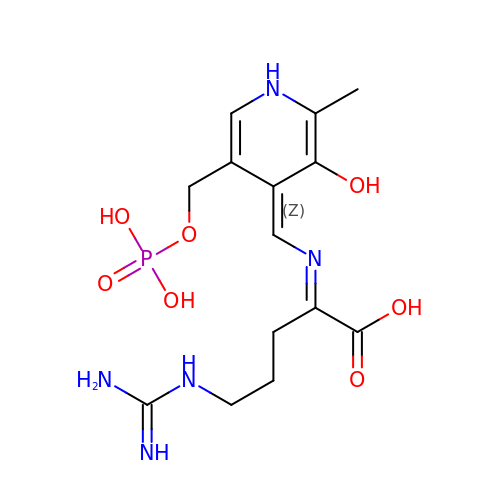(2E)-5-carbamimidamido-2-{[(Z)-{3-hydroxy-2-methyl-5-[(phosphonooxy)methyl]pyridin-4(1H)-ylidene}methyl]imino}pentanoic acid | C14 H22 N5 O7 P | RHCMSTSZICWJMS-GXVFZPQQSA-N> SPGQGTQSENSCTHFPGNLPNMLRDLRDAFSRVKTFFQMKDQLDNLLLKESLLEDFKGYLGCQALSEMIQ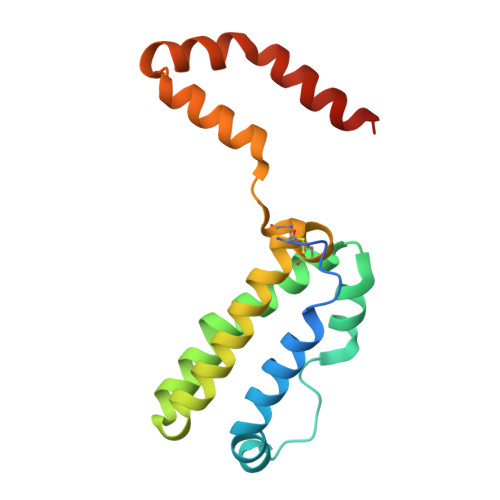FYLEEVMPQAENQDPDIKAHVNSLGENLKTLRLRLRRCHRFLPCENKSKAVEQVKNAFNKLQEKGIYKAMSEFDIFINYIEAYMTMKIRN> GSHFYFLSKRRRNLLRNPCGEEDLEGWSDVEHGGDGWKVEELPGDNGVEFTQDDSVKKYFASSFEWCRKAQVIDLQAEGYWEELLDTTQPAIVVKDWYSGRTDAGSLYELTVRLLSE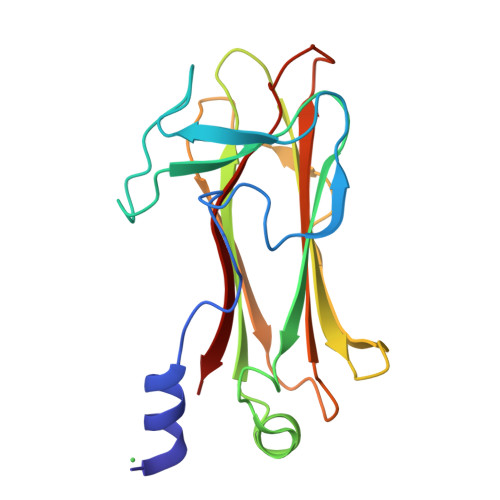NEDVLAEFATGQVAVPEDGSWMEISHTFIDYGPGVRFVRFEHGGQDSVYWKGWFGARVTNSSVWVEP>[9x]PDVPKGCEGPCKVQSYEQRHDISHVGKVLCVSDVTRGNGLTHRVGKRFCVKSVYVLGKIWMDENIKTKNHTNTVMFYLVRDRRPFGTAMDFGQVFNMYDNEPSTATIKNDLRDRYQVLRKFTSTVTGGQYASKEQALVKKFMKINNYVVYNHQEAAKYDNHTENALLLYMACTHASNPVYATLKIRIYFYDSVQN;> NRRRTWTNRPMYRKPRLYRMYRTPDVPKGCEGPCKVQSYEQRHDISHVGKVLCVSDVTRGNGLTHRVGKRFCVKSVYVLGKIWMDENIKTKNHTNTVMFYLVRDRRPFGTAMDFGQVFNMYDNEPSTATIKNDLRDRYQVLRKFTSTVTGGQYASKEQALVKKFMKINNYVVYNHQEAAKYDNHTENALLLYMACTHASNPVYATLKIRIYFYDSVQN;> RLYRMYRTPDVPKGCEGPCKVQSYEQRHDISHVGKVLCVSDVTRGNGLTHRVGKRFCVKSVYVLGKIWMDENIKTKNHTNTVMFYLVRDRRPFGTAMDFGQVFNMYDNEPSTATIKNDLRDRYQVLRKFTSTVTGGQYASKEQALVKKFMKINNYVVYNHQEAAKYDNHTENALLLYMACTHASNPVYATLKIRIYFYDSVQN

Whereas nanoviruses have T = 1 icosahedral capsids of ~18 nm in diameter (although no detailed structures are available), geminiviruses are formed from two such isometric particles, or ‘hemicapsids’, fused to form a geminate particle (18 × 30 nm) which gives the virus family its name. Here we present the cryo-EM structure of AYVV at 3.3 Å resolution. The structure shows that the capsid is built from three distinct conformations of a single CP, and that these conformational differences facilitate the formation of the interface between hemicapsids. The body of the CP is similar to that of STNV and many other viruses, consisting of a jelly-roll fold with two twisted, 4-stranded β-sheets.

Structure refinement with D5 symmetry, yielded a density map at 3.3 Å resolution, and an atomic model for the CP layer was built and refined, starting from a homology model of the STNV CP. The capsid is composed of 110 copies of the CP, and we built and refined a complete D5 asymmetric unit of 11 unique chains (chains A-K). Each hemicapsid is formed from a T = 1 particle from which a penton of CP subunits is missing. The different conformations needed to build a geminivirus arise through differences in the N-terminal domain of the CP, rather than in its core fold. The biggest change is in subunit H, where an extra 23 residues are resolved as a helix-loop-helix motif (first ordered residue: 40). By contrast in chain I, an extra 8 residues (first ordered residue: 55) become ordered, but in an extended conformation that is different to that seen for the same residues in chain H. The helix-loop-helix motif from chain H is a major component of the equatorial interface, making a series of H-bonding interactions to a patch of predominantly polar residues in the body of the CP subunit across the interface (residues 214 & 215 in chain I), which is surrounded by van der Waals interactions. The ordered segment from chain I extends across to stabilize the base of the helix-loop-helix motif in an adjacent H subunit, presumably stabilizing the ring of equatorial subunits. The map was of sufficient quality to build 7 nucleotides into the density beneath each subunit, except for subunit H at the interface where there are 6. More significantly, a new interaction occurs between the backbone of nucleotide 5 and R41, at the extreme N-terminus of the helix-loop-helix motif in chain H. This motif forms the equatorial interface, and presumably the interaction with DNA stabilizes this structural element.> KTNLANEDEAYEAIFG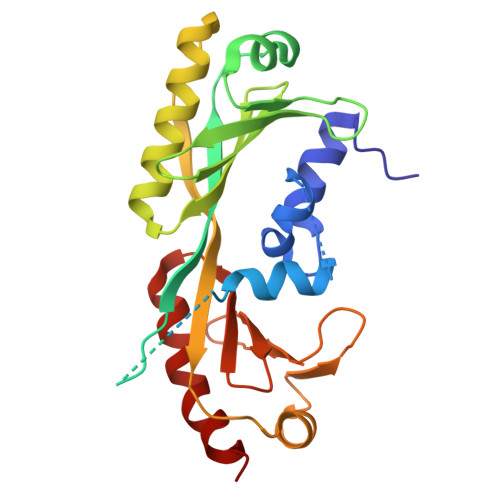GEFGSLEIGSYIGGDEGGGSADQLEMVTELLGGDMVNQSFICDPDDETFIGGGSGGGSGGGSMSGIVPTLQNIVATVTLGCRLDLKTVALHARNAEYNPKRFAAVIMRIREPKTTALIFASGKMVVTGAKSEDDSKLASRKYARIIQKIGFAAKFTDFKIQNIVGSCDVKFPIRLEGLAFSHGTFSSYEPELFPGLIYRMVKPKIVLLIFVSGKIVLTGAKQREEIYQAFEAIYPVLSEFRKM> UGCUXCUAGUACG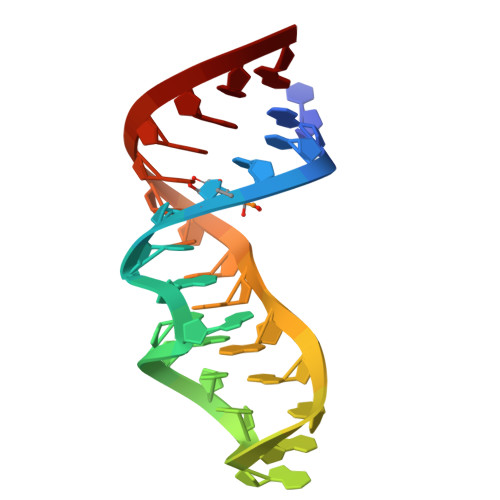AGAGGACCGGAGUG>AMAEMKTDAATLAQEAGNFERISGDLKTQIDQVESTAGSLQGQWRGAAGTAAQAAVVRFQEAANKQKQELDEISTNIRQAGVQYSRADEEQQQALSSQMGF[2x]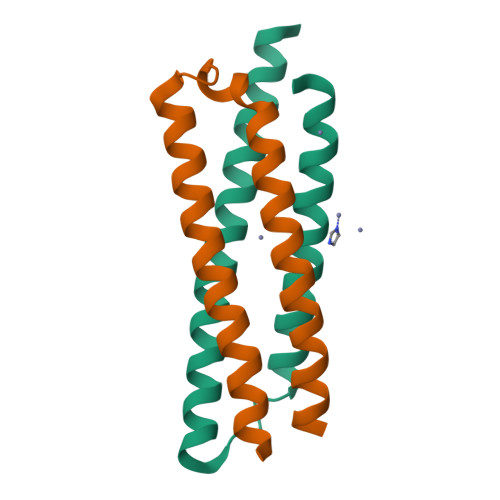;>[2x]TEQQWNFAGIEAAASAIQGNVTSIHSLLDEGKQSLTKLAAAWGGSGSEAYQGVQQKWDATATELNNALQNLARTISEAGQAMASTEGNVTGMFA> MGSSHHHHHHHSSGRENLYFQGHMEGVRWAFSCGTWLPSRAEWLLAVRSIQPEEKERIGQFVFARDAKAAMAGRLMIRKLVAEKLNIPWNHIRLQRTAKGKPVLAKDSSNPYPNFN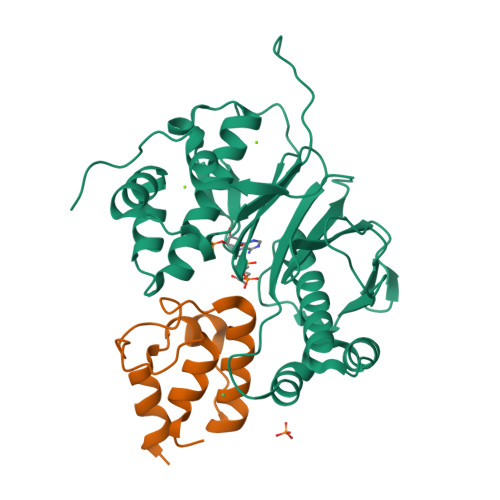FNISHQGDYAVLAAEPELQVGIDIMKTSFPGRGSIPEFFHIMKRKFTNKEWETIRSFKDEWTQLDMFYRNWALKESFIKAIGVGLGFELQRLEFDLSPLNLDIGQVYKETRLFLDGEEEKEWAFEESKIDEHHFVAVALRKPDGSRHQDVPSQDDSKPTQRQFTILNFNDLMSSAVPMTPEDPSFWDCFCFTEEIPIRNGTKS;> GTRDRDSQRDLVEAVAHILGIRDLAAVNLDSSLADLGLDALMSVEVRQTLERELNLVLSVREVRQLTLRKLQELSSKADEASELACPTPKE>[6x]SNAMSEDNYRTIALAFLDESADSTTINAWVNEFA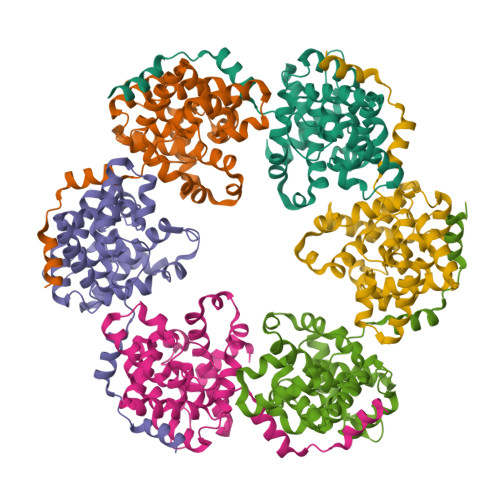YQGFDPKRIVQLVKERGTAKGRDWKKDVKMMIVLNLVRGNKPESMMKKMSEKGAAIVTQLISTYQLKEGNPGRDTITLSRVSAAFVPWTVQALKTLSESLPVTGTTMDSIAGTTYPRCMMHPSFAGIIDLELPNNTGAMLADAHGLFMLEFSKTINPSLRTKQPNEIAATFEKPNMAAMTGRFFTRDDKKKLLIAIGVLNEDLVPNPAIEKCAEKYKAKVGKV>[8x]MTQCYAEITGWGKCLPPATLSNHDLSTFLDTSDEWIQSRTGIEQRRISHVNTSDLATVAAQHAIACAGVSVEEIDLIIVATCSPDSLIPNIASRVQQNLGIPSAAAFDLNAACTGFLYGLETATRLMQASHYRHALVIGAERLSFYLDWTKRDTAVLFGDGAGAVVLSKTEQKVGLQDAQIGCDAQGRDILAVPKFGTAMDRFDADNGYWAFDFVGK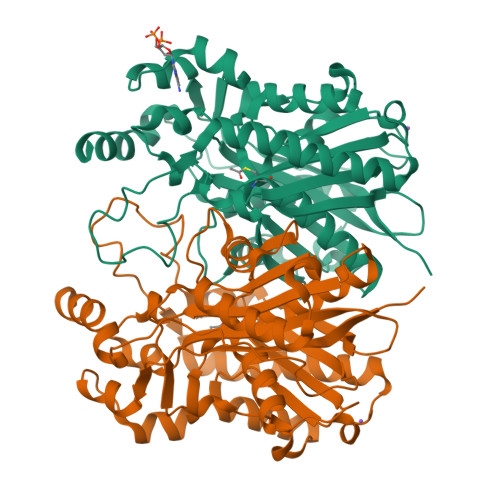EIFKRAVRGMGAAAQQVLARSGLSTEEIDVVIPHQANIRIIQTLCDLAGIAQDKAFVNIHRYGNTSAATVPIALCEALEQGKIKPHDDLLVAAFGAGLTWGAGHIRWGERITPLGKSDAQLPSCDHTALDLLSKAIEHCKRHQSE>[2x]EA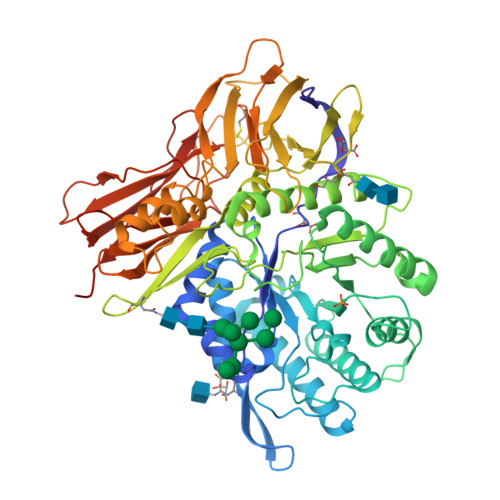PHLVHVDAARALWPLRRFWRSTGFCPPLPHSQADQYVLSWDQQLNLAYVGAVPHRGIKQVRTHWLLELVTTRGSTGRGLSYNFTHLDGYLDLLRENQLLPGFELMGSASGHFTDFEDKQQVFEWKDLVSSLARRYIGRYGLAHVSKWNFETWNEPDHHDFDNVSMTMQGFLNYYDACSEGLRAASPALRLGGPGDSFHTPPRSPLSWGLLRHCHDGTNFFTGEAGVRLDYISLHRKGARSSISILEQEKVVAQQIRQLFPKFADTPIYNDEADPLVGWSLPQPWRADVTYAAMVVKVIAQHQNLLLANTTSAFPYALLSNDNAFLSYHPHPFAQRTLTARFQVNNTRPPHVQLLRKPVLTAMGLLALLDEEQLWAEVSQAGTVLDSNHTVGVLASAHRPQGPADAWRAAVLIYASDDTRAHPNRSVAVTLRLRGVPPGPGLVYVTRYLDNGLCSPDGEWRRLGRPVFPTAEQFRRMRAAEDPVAAAPRPLPAGGRLTLRPALRLPSLLLVHVCARPEKPPGQVTRLRALPLTQGQLVLVWSDEHVGSKCLWTYEIQFSQDGKAYTPVSRKPSTFNLFVFSPDTGAVSGSYRVRALDYWARPGPFSDPVPYLEVPVPRGPPSPGNP> MGMPSGWELLLVVGVIVLLFGGKKIPELAKGLGKG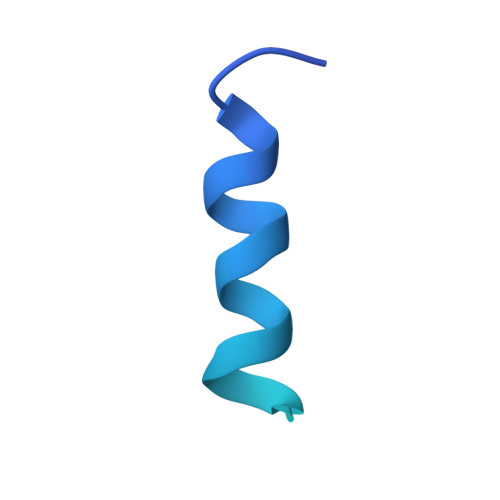IKDFKQAVKEDEEASAPAKEIENKEASASGTQSEASEVKESQKAWSHPQFEK> MFPSPRAQGMGSARRPFNSRLTGGRKALGPGVTASSSPSALYSPVGRRVSASGARSTPSRVYLHPAASETVNYNVQLFGSSLPVKVMEALSNASADEPMAACIHEGGWAWLACNDRLIIWKISHSSSAKLMVCKELPLPLSDSEWSADLVDICAQTGDPAAAQSVALMAATPEGSSRYWPNILHEGTYIESYTEFGSSLCAFVTAVKGNSFILSSEKNQLVRLTPDASGKMNQRVLPQGQGMLSGIGRRVSTLFGILSPAVESTLCSVLWDKGDCFYTLTDSSINKWDLDDTSESQVLNWDMSRVLREYISDAIWGSESDYDDIKAGININYLSLNQNCDGLVILSAAWHPGDNPCQIYYTLVTVKDEGYNISDEITVEVTQFNPVFQARGMQLCQLVVPNFSSQACYLYTQEMIFACSTGTGRSTLPQEKIPFEAQGDNIVGAGSCEGWPVFFIRKSGMLTVVARETASVLPEHMEESLSSVSKSSRQAVVKDSRPDQIAHDDKTKHLKAAFLRYCRKDILGAQSMVDSLFSDSDMEPDDELDLAVNQISVDLIDDYPASDPRWAESVPEEAAGFSNTSLILLHQLEDKMKAHSFFVDFLHQVGLFSRLSTCQTKGMLVATRLLLSEHAEKLSAAIVLKNHHAKLPVLVNSAIQLALDKRMCTVPQNLTAADVYFREVSQMEIIFECLVDKEEADLESTSIDSVEWANIVVNVNTILKDMLHVACQYRQSKNSLYKNESGIQEPEHVPWTASSGTAGIRSVVTRQHGIILKVYPQADSGLRTILIEQLAALLNYLLDDYVTQLKSIDKLANEERYNILEMEYAQKRSELLSPLLILGQYAWASNLAEKYCDFDILVQICEMTDNQSRLQRYMTLFAEQNFSDFLFRWYLEKGKRGKLLSQPASQHGQLAAFLQAHDHLSW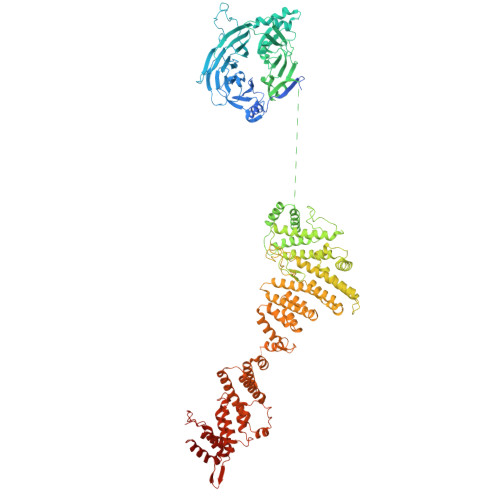LHELNSQEFEKAHRTLQTLANMETRYFCKKKTLLGLSKLAALASDFQEDVLQEKVEEIAEQEHFLLHQETLPKKLLEEKQLDLNAMPVLAPFQLIQLYVCEENKRANENDFMKALDLLEYIGDDSEVDVEELKLEILCKAIKRDEWSATDGKDDPIEATKDSIFVKVLQNLLNKGIELKGYLPKAETLLQSEELNSLKTNSYFEFSLKANYECYMKMQS>SNAMKNYYSSNPTFYLGIDCIIFGFNEGEISLLLLKRNFEPAMGEWSLMGGFVQKDESVDDAAKRVLAELTGLENVYMEQVGAFGAIDRDPGERVVSIAYYALININEYDRELVQKHNAYWVNINELPALIFDHPEMVDKAREMMKQKA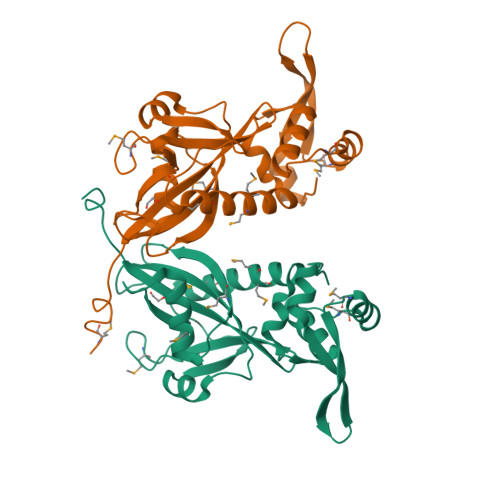SVEPIGFNLLPKLFTLSQLQSLYEAIYGEPMDKRNFRKRVAEMDFIEKTDKIDKLGSKRGAALYKFNGKAYRKDPKFKL[4x]> AQSVPYGVSQIKAPALHSQGYTGSNVKVAVIDSGIDSSHPDLKVAGGASMVPSETNPFQDNNSHGTHVAGTVAALNNSIGVLGVAPSASLYAVKVLGADGSGQYSWIINGIEWAIANNMDVINMSLGGPSGSAALKAAVDKAVASGVVVVAAA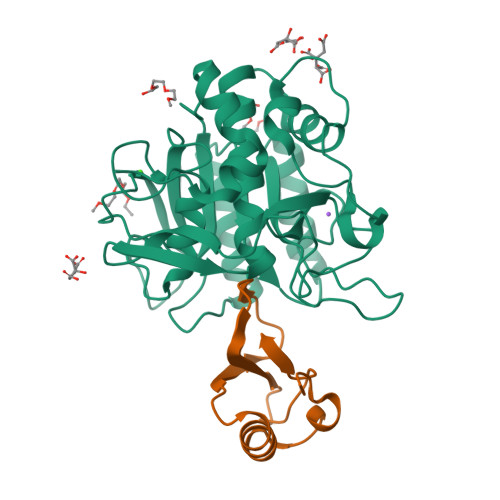GNEGTSGSSSTVGYPGKYPSVIAVGAVDSSNQRASFSSVGPELDVMAPGVSIQSTLPGNKYGAYNGTSMASPHVAGAAALILSKHPNWTNTQVRSSLENTTTKLGDSFYYGKGLINVQAAAQHHHHHH;> MKTEWPELVGKSVEEAKKVILQDKPAAQIIVLPVGTIVPMEYRIDRVRLFVDRLDNIAQVPRVG>METSENKSEIKILSLNGGGVRGLFTITLLAELESIIEKREKCENVKIGDYFDLITGTSIGGILALGLASGKSARELKEAFEINATKIFPLKRFKNKQWWNLLRRSIYESEPLYDAVKSMIGETIKFEDLNRRVMITSVNLSTGKPKFFKTPHNPMFTMDREIRLIDAAMATSAAPTYFKPHYIEKLENYFADGGLVANNPSYIGIREVLIDMKNDFPDAKPENIKVLNIGTLSEDYCISPETLSKNSGKGYLSLWNMGERIVLSTMTANQHLQRFMLLREFEALKIEKNYVEIDETIPNEAAAEITLDNASEGCLKALRGSGKKLAAERYTKNEELR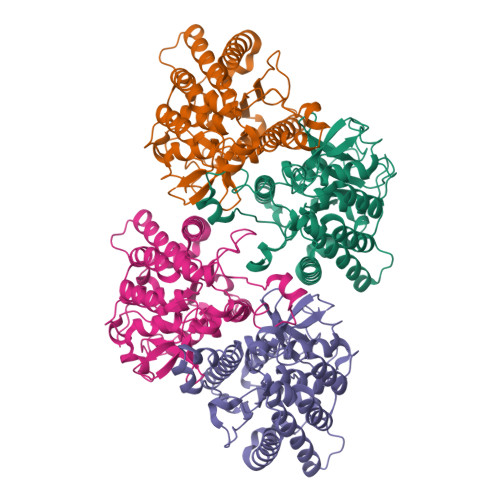NFFLKKAEPFVPYIESSEVTAHHHHHH[4x]> MNSKHSYVELKDKVIVPGWPTLMLEIDFVGGTSRNQFLNIPFLSVKEPLQLPREKK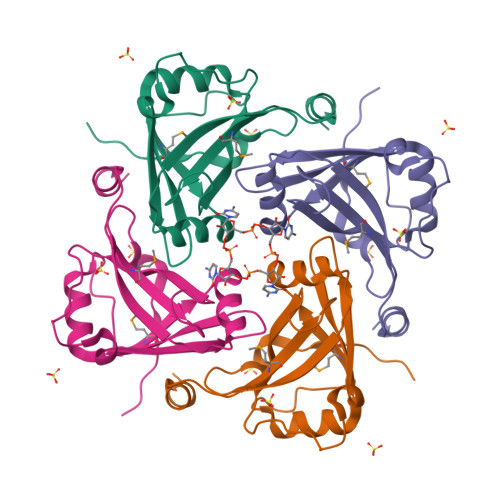LTDYFTIDVEPAGHSLVNIYFQIDDFLLLTLNSLSVYKDPIRKYMFLRLNKEQSKHAINAAFNVFSYRLRNIGVGPLGPDIRSSGP>[36x]MGNRGMEDLIPLVNRLQDAFSAIGQNADLDLPQIAVVGGQSAGKSSVLENFVGRDFLPRGSGIVTRRPLVLQLVNATTEYAEFLHCKGKKFTDFEEVRLEIEAETDRVTGTNKGISPVPINLRVYSPHVLNLTLVDLPGMTKVPVGDQPPDIEFQIR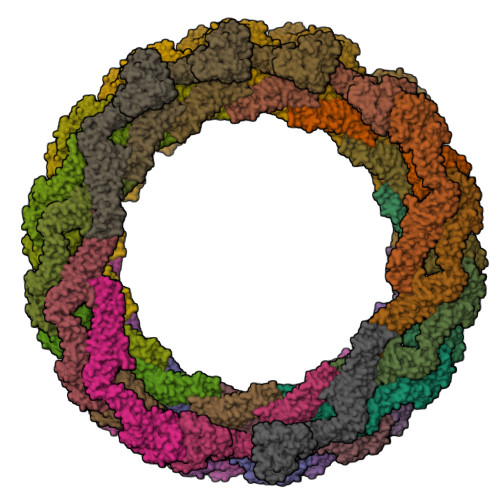DMLMQFVTKENCLILAVSPANSDLANSDALKVAKEVDPQGQRTIGVITKLDLMDEGTDARDVLENKLLPLRRGYIGVVNRSQKDIDGKKDITAALAAERKFFLSHPSYRHLADRMGTPYLQKVLNQQLTNHIRDTLPGLRNKLQSQLLSIEKEVEEYKNFRPDDPARKTKALLQMVQQFAVDFEKRIEGSGDQIDTYELSGGARINRIFHERFPFELVKMEFDEKELRREISYAIKNIHGIRTGLFTPDMAFETIVKKQVKKIREPCLKCVDMVISELISTVRQCTKKLQQYPRLREEMERIVTTHIREREGRTKEQVMLLIDIELAYMNTNHEDFIGFANAQQRSNQMNKKKTSGNQDEILVIRKGWLTINNIGIMKGGSKEYWFVLTAENLSWYKDDEEKEKKYMLSVDNLKLRDVEKGFMSSKHIFALFNTEQRNVYKDYRQLELACETQEEVDSWKASFLRAGVYPERVGDKEKASETEENGSDSFMHSMDPQLERQVETIRNLVDSYMAIVNKTVRDLMPKTIMHLMINNTKEFIFSELLANLYSCGDQNTLMEESAEQAQRRDEMLRMYHALKEALSIIGNINTTTVSTPMPPPVDDSWLQVQSVPAGRRSPTSSPTPQRRAPAVPPARPGSRGPAPGPPPAGSALGGAPPVPSRPGASPDPFGPPPQVPSRPNRAPPGVPSRSGQASPSRPESPRPPFDL>[2x]GSKKHTGYVGLKNQGATCYMNSLLQTLFFTNQLRKAVYMMPTEGDDSSKSVPLALQRVFYELQHSDKPVGTKKLTKSFGWETLDSFMQHDVQELCRVLLDNVENKMKGTCVEGTIPKLFRGKMVSYIQCKEVDYRSDRREDYYDIQLSIKGKKNIFESFVDYVAVEQLDGDNKYDAGEHGLQEAEKGVKFLTLPPVLHLQLMRFMYDPQTDQNIKINDRFEFPEQLPLDEFLQ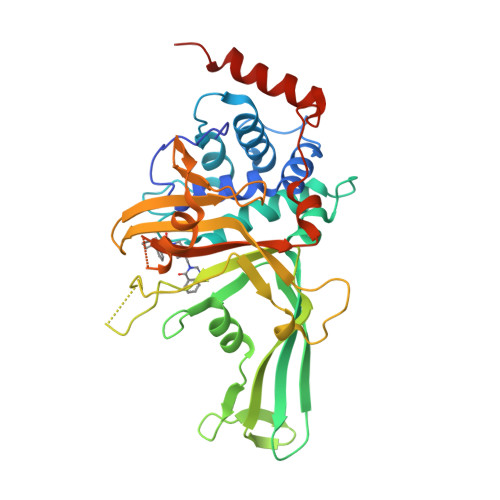KTDPKDPANYILHAVLVHSGDNHGGHYVVYLNPKGDGKWCKFDDDVVSRCTKEEAIEHNYGGHDDDLSVRHCTNAYMLVYIRESKLSEVLQAVTDHDIPQQLVERLQEEKRIEAQKRKERQE>[4x]MASMTGMPNYNIPFSPPDITEAEITEVVDTLRSGWITTGPKTKELERRLSLYTQTPKTVCLNSATAALELILRVLEVGPGDEVIVPAMTYTASCSVITHVGATPVMVDIQADTFEMDYDLLEQAITEKTKVIIPVELAGIVCDYDRLFQVVEKKRDFFTASSKWQKAFNRIVIVSDSAHALGSTYKGQPSGSIADFTSFSFHAVKNFTTAEGG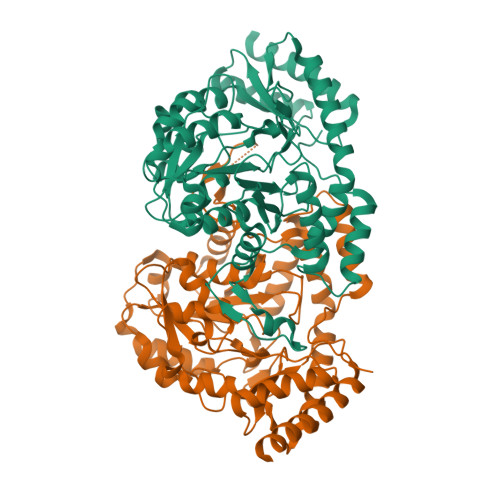SATWKANPVIDDEEMYKEFQILSLHGQTKDALAKMQLGSWEYDIVTPAYKCNMTDIMASLGLVQLDRYPSLLQRRKDIVDRYDSGFAGSRIHPLAHKTETVESSRHLYITRVEGASLEERNLIIQELAKAGIASNVHYKPLPLLTAYKNLGFDMTNYPKAYAFFENEITLPLHTKLSDEEVDYIIETFKTVSEKVLTLSKKKLAAALEHHHHHH>[6x]RAGKNPREEILDASAELFTRQGFATTSTHQIADAVGIRQASLYYHFPSKTEIFLTLLKST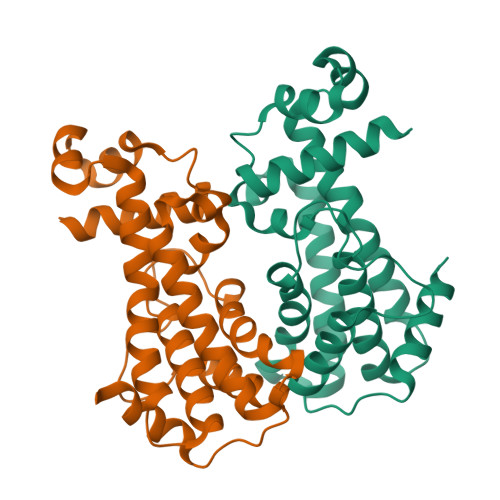VEPSTVLAEDLSTLDAGPEMRLWAIVASEVRLLLSTKWNVGRLYQLPIVGSEEFAEYHSQREALTNVFRDLATEIVGDDPRAELPFHITMSVIEMRRNDGKIPSPLSADSLPETAIMLADASLAVLGAPLPADRVEKTLELIKQADAK> GHWDGGAEKAD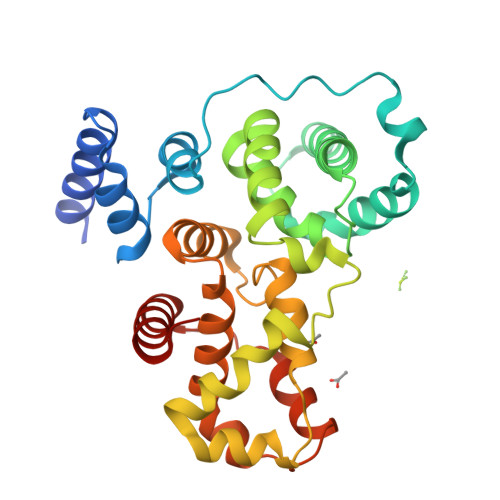FNAKRKKKVAEIHQALNSDPTDVAALRRMAISEGGLLTDEIRRKVWPKLLNVNANDPPPISGKNLRQMSKDYQQVLLDVRRSLRRFPPGMPEEQREGLQEELIDIILLILERNPQLHYYQGYHDIVVTFLLVVGERLATSLVEKLSTHHLRDFMDPTMDNTKHILNYLMPIIDQVNPELHDFMQSAEVGTIFALSWLITWFGHVLSDFRHVVRLYDFFLACHPLMPIYFAAVIVLYREQEVLDCDCDMASVHHLLSQIPQDLPYETLISRAGDLFVQFPPS>[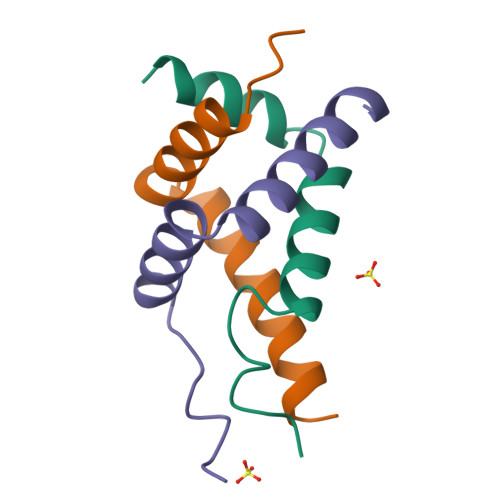6x]GPHMADLLLNSTQFVQAFTYLIQNDKEFANKLHKAYLNGCSNLLLD> KPVSLSYRCPCRFFESHVARANVKHLKILNTPNCALQIVA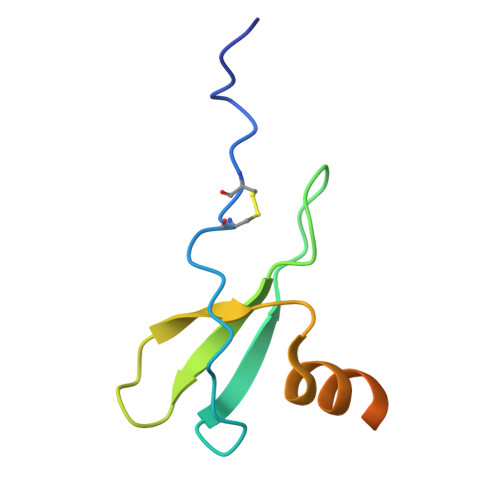RLKNNNRQVCIDPKLKWIQEYLEKALNKRFKMHHHHHHHH> GAGSMLVLITYDVQTSSMGGTKRLRKVAKACQNYGQRVQNSVFECI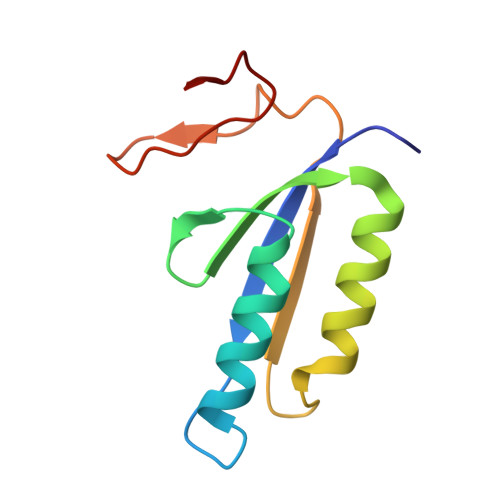VDSTQLTSLKLELTSLIDEEKDSLRIYRLGNNYKTKVEHIGAKPSIDLEDPLIF> 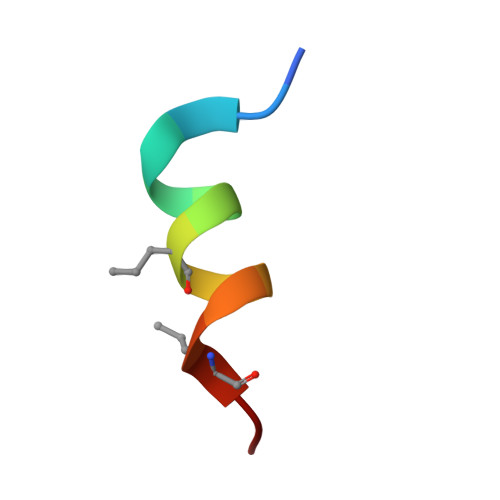KETAAAKVERQHLDS> MKTNPGRFFEDFRLGETIRHATPRTVTTGDVALYTALYGPRFTVQSSDAFAKTIGYPASPLDDLLTFHVVFGKTVPDVSLNALANLGYAEGGFHRPVYPGETLSTVSEVIGLKESSNRQTGVVYVRSTGSDASGRTVLSYCRWVLVRKRDPEAKIAEEHVPQLAKVVNPADLAHALPPLDPAAYDNALAGSPHRFADYAVGEKIDHVDGMTVEEAEHQIATRLFQNTAKVHFDAVATKETKFGKRLIYGGHVISLARALSFNGLANAFAIGGINAGRHVAPLFAGDTVYAWSEVLETAELPGRSDIGALRLRTVATKNQACGAYPDKQGEGYDPSVILDLDYWAFIPRLEHHHHHH

In this study, we determined the crystal structure of the mesaconyl-CoA hydratase from M. extorquens (MeMeaC) that catalyzes the reversible conversion of mesaconyl-CoA to β-methylmalyl-CoA. MeaC functions as a mesaconyl-CoA hydratase, reversibly catalyzing mesaconyl-CoA into β-methylmalyl-CoA, by adding one water molecule. The crystal structure of MeMeaC revealed that the enzyme belongs to the MaoC-like dehydratase domain superfamily and functions as a trimer. The ethylmalonyl-CoA pathway is an anaplerotic reaction sequence essential for the assimilation of acetyl-CoA, which is necessary for methylotrophic growth.

To elucidate the molecular mechanism and substrate binding mode of MeMeaC, we determined the crystal structure of the enzyme at a 1.95 Å resolution with Rwork = 20.9% and Rfree = 27.8%, respectively. MeMeaC is composed of an N-terminal subdomain (MeaCN, residue 1~147), a C-terminal subdomain (MeaCC, residue 191~348), and a bridge (MeaCBr, residue 148~190) linking the two subdomains. Although one molecule is present in the asymmetric unit of the crystal structure, the P63 crystallographic symmetry operation of MeMeaC revealed that the enzyme forms a trimer. In our current structure of MeMeaC, we observed that a malic acid molecule, which is used as a main precipitant for the crystallization, is bound at the active site. The binding site of the malic acid molecule is formed at the interface between MeaCN and MeaCC. The conserved residues, such as Phe71, Ser79, Asn85, Arg142, Asn226, His231, Tyr248, and Gly249, were located at the malic acid binding site. Oxygen of Ser79 sidechain and nitrogen of Arg142 sidechain make hydrogen bonds to O1 and O2 of malic acid with 2.6 Å and 2.8 Å distances. Nitrogen atoms of Asn85 and Gly249 backbones form hydrogen bonds to O4 and O5 of malic acid with 2.6 Å and 3.0 Å distances. O3 of malic acid interacts with nitrogen atoms of sidechains of Asn226 and His231 as hydrogen bonds of 2.6 Å and 3.0 Å distances. Taking into account that a β-methylmalyl-CoA has an additional hydroxyl group at the counterpart of O3 of the malic acid and is not at a mesaconyl-CoA, strong interaction of Asn226–O3–His231 could make the binding of a β-methylmalyl-moiety more stable, which contributes to improving the specificity.Human ATP-binding cassette transporter subfamily B6 (ABCB6) is a mitochondrial porphyrin transporter that uses energy from ATP hydrolysis to translocate the heme precursors protoporphyrin IX and coproporphyrinogen III from the cytoplasm into mitochondria for heme biosynthesis. ABCB6 is a Type IV half-transporter of 842 amino acids with only one transmembrane domain (TMD) and one cytosolic nucleotide-binding domain (NBD) with an extra N-terminal TMD (TMD0). It functions as a homodimer with the substrate transport pathway and the active site of ATP hydrolysis built from residues from both chains. Within the transport pathway, a conserved aromatic residue W546 located in each monomer plays a pivotal role in stabilizing the occluded conformation via π-stacking interactions.

To evaluate the structural impact of W546A mutation, we prepared grids using detergent-purified or nanodisc-reconstituted W546A mutant. As expected, the first 3D classification analysis revealed that most of the detergent-purified mutant molecules (59.5%) adopted an outward-facing conformation (and Supplementary Figs. 6−8). The final EM density map of the detergent-purified W546A mutant in the outward-facing state was obtained from the best 3D class containing 56,293 particles at a resolution of 3.9 Å with C1 or C2 symmetry, which enabled us to build an almost complete model of the transporter. The structure has the typical features expected for the outward-facing conformation of an ABC transporter. The TMDs form a V-shaped translocation pathway that is both open to the extracellular space and laterally to the membrane outer leaflet. There was no density corresponding to CPIII, suggesting that the bound substrate is exported from the transporter prior to ATP hydrolysis and ADP/Pi release. However, the structure has relatively poor electron density and high B-factors for the extracellular side of TMDs, suggesting that these regions undergo highly dynamic motions to promote substrate release. In the NBD dimer, the two Mg2+/ADP·VO4 molecules are sandwiched at the interface, interacting with the Walker A and B motifs, the A- and Q-loop residues of one NBD, and the ABC signature motif (LSGGE) of the opposing NBD. However, adoption of the outward-facing conformation exposes negatively-charged residues E346, D374, E446, and E487 at the bottom of the cavity. This negatively-charged surface appears to promote substrate release into the extracellular space by pushing porphyrins along the translocation pathway via charge repulsion, while simultaneously preventing exported substrates from re-entering the cavity. Conversely, adoption of an outward-facing conformation shifts the side chains of key residues away from the substrate-binding site (lower right).

>[2x]RDFGRKLRLLSGYLWPRGSPALQLVVLICLGLMGLERALNVLVPIFYRNIVNLLTEKAPWNSLAWTVTSYVFLKFLQGGGTGSTGFVSNLRTFLWIRVQQFTSRRVELLIFSHLHELSLRWHLGRRTGEVLRIADRGTSSVTGLLSYLVFNVIPTLADIIIGIIYFSMFFNAWFGLIVFLCMSLYLTLTIVVTEWRTKFRRAMNTQENATRARAVDSLLNFETVKYYNAESYEVERYREAIIKYQGLEWKSSASLVLLNQTQNLVIGLGLLAGSLLCAYFVTEQKLQVGDYVLFGTYIIQLYMPLNAFGTYYRMIQTNFIDMENMFDLLKEETEVKDLPGAGPLRFQKGRIEFENVHFSYADGRETLQDVSFTVMPGQTLALVGPSGAGKSTILRLLFRFYDISSGCIRIDGQDISQVTQASLRSHIGVVPQDTVLFNDTIADNIRYGRVTAGNDEVEAAAQAAGIHDAIMAFPEGYRTQVGERGLKLSGGEKQRVAIARTILKAPGIILLDEATSALDTSNERAIQASLAKVCANRTTIVVAHRLSTVVNADQILVIKDGCIVERGRHEALLSRGGVYADMWQLQQ>[2x]SMVRTEPFQDGYSLCPGRELGRGKFAVVRKCIKKDSGKEFAAKFMRKRRKGQDCRMEIIHEIAVLELAQDNPWVINLHEVYETASEMILVLEYAAGGEIFDQCVADREE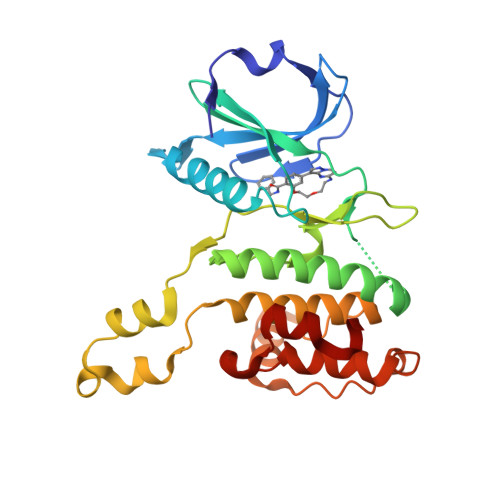AFKEKDVQRLMRQILEGVHFLHTRDVVHLDLKPQNILLTSESPLGDIKIVDFGLSRILKNSEELREIMGTPEYVAPEILSYDPISMATDMWSIGVLTYVMLTGISPFLGNDKQETFLNISQMNLSYSEEEFDVLSESAVDFIRTLLVKKPEDRATAEECLKHPWLT> PGVERTDITYNLTSDIDAAAYLEELKQNPIINNKIMNPVGQCESLMTPVSNFMNEKGFDNIRYRGIFIWDKPTEEIPTNHFAVVGNKEGKDYVFDVSAHQFENRGMSNLNGPLILSADEWVCKYRMATRRKLIYYTDFSNSSIAANAYDALPRELESESMAGKVFVTSPRWFNTFKKQKYSLIGKM

SseI is secreted into host cells by Salmonella and contributes to the establishment of systemic infections. SseI (also called SrfH) is an SPI-2-translocated protein that has been directly linked to systemic infection. The C-terminal domain (∼140–322) of SseI contains its catalytic function and shows some sequence similarity (19% identity over a 88-amino-acid stretch) to Pasteurella multocida toxin (PMT or ToxA), which causes atrophic rhinitis in swine. Based on its structural matches, SseI is a member of a particular subgroup (clan CA) of the cysteine protease superfamily.

In this work, we were able to determine the domain organization of SseI and obtain a crystal structure of its catalytic C-­terminal domain (reductively methylated; residues 137–322) by SAD to 1.70 Å resolution. The overall structure and topology of the high-resolution (1.7 Å) SeMet-derivative structure revealed a single catalytic domain consisting of a core of six antiparallel β-sheets and eight surrounding helices. No density was observed for 12 residues at the N-terminus (137–144 and four vector-encoded residues), nine residues at the C-­terminus (314–322) or for residues 264–266 (a presumed disordered loop). The SeMet protein was purified using 10 mM DTT instead of 2 mM DTT to prevent Se oxidation, which may explain why it did not crystallize as a disulfide-linked dimer under these reducing conditions. It might also be the reason why seeding was not required to obtain large diffracting crystals of the SeMet protein. The higher resolution SeMet-derivative structure was used for all subsequent structural analyses. The SseI structure shows significant similarity to those of members of the cysteine protease superfamily, which allowed the identification of the catalytic triad: Cys178, His216 and Asp231. The measured Cys-to-His (3.5 Å) and His-to-Asp (2.8 and 3.4 Å) bond distances fit well to those expected for this type of catalytic triad. There is no room in this cavity for additional molecules and there are no other cavities from the surface that lead towards the active-site residues, making it likely that a small molecule such as water is involved in the catalytic mechanism of SseI. Looking at the region surrounding the active site, it is not obvious what type of substrate would be likely to bind, as there is both a positively charged and a negatively charged region on opposite sides of the solvent-accessible Cys178.>[4x]GSMGSKKLTVGSDSHRLSKSSFSSNKSSHSATKDQPIDTDDIDEDDESGHNIILNI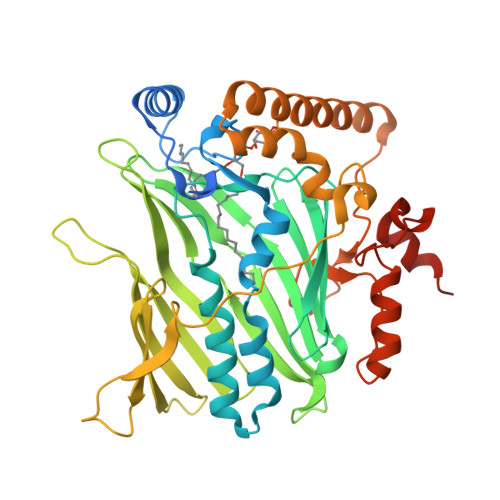ISQLRPGCDLTRITLPTFILEKKSMLERVTNQLQFPEFLLQAHSEKDPLKRFLYVMKWYLAGWHIAPKAVKKPLNPVLGEYFTAYWDLPNKQQAYYISEQTSHHPPECAYFYMIPESSIRVDGVVIPKSRFLGNSSAAMMDGSTVLQFLDIKDGNGKPEKYVLTQPNVYVRGILFGKMRIELGDHMIIKSPNFQADIEFKTKGYVFGTYDAIEGTVKDYDGNAYYEISGKWNDVMYLKDLKQPRSSPKVFLDTHKESPLRPKVRPLSEQGEYESRKLWKKVTDALAVRNHPVATEEKFQIEDHQRQLAKKRIEDGVEFHPKLFRRSKPGEDLDYCIYKNIPVDEDPEKQIRSILQIAPILPGQQFTDKFFIPAFEKIKSQKKMIENEKQNPAKQ>KPGAPWWKSAVFYQVYPRSFKDTNGDGIGDFKGLTEKLDYLKGLGIDAIWINPHYASPNTDNGYDISDYREVMKEYGT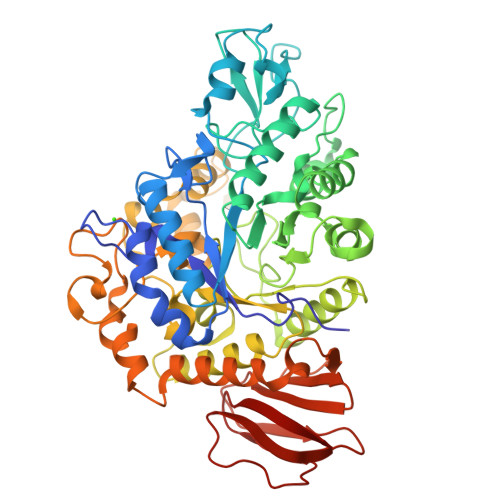MEDFDRLMAELKKRGMRLMVDVVINHSSDQHEWFKSSRASKDNPYRDYYFWRDGKDGHEPNNYPSFFGGSAWEKDPVTGQYYLHYFGRQQPDLNWDTPKLREELYAMLRFWLDKGVSGMRFATVATYSKTPGFPDLTPEQMKNFAEAYTQGPNLHRYLQEMHEKVFDHYDAVTAGEIFGAPLNQVPLFIDSRRKELDMAFTFDLIRYDRALDRWHTIPRTLADFRQTIDKVDAIAGEYGWNTFFLGNHDNPRAVSHFGDDRPQWREASAKALATVTLTQRGTPFIFQGDELGMTNYPFKTLQDFDDIEVKGFFQDYVETGKATAEELLTNVALTSRNNARTPFQWDDSANAGFTTGKPWLKVNPNYTEINAAREIGDPKSVYSFYRNLISIRHETPALSTGSYRDIDPSNADVYAYTRSQDGETYLVVVNFKAEPRSFTLPDGMHIAETLIESSSPAAPAAGAASLELQPWQSGIYKVK[2x]>[2x]SNASKMSDVKCTSV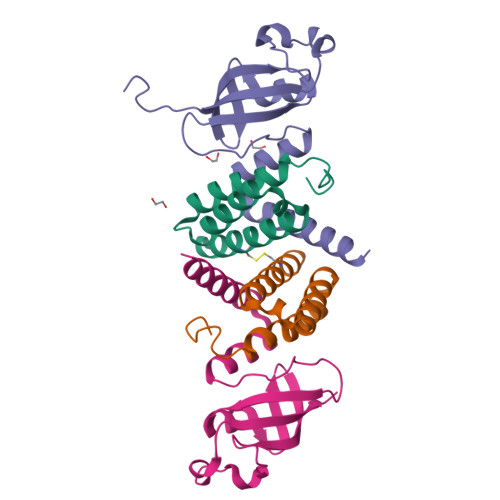VLLSVLQQLRVESSSKLWAQCVQLHNDILLAKDTTEAFEKMVSLLSVLLSMQGAVDINKLCEEMLDNRATLQ;>[2x]EDKRAKVTSAMQTMLFTMLRKLDNDALNNIINNARDGCVPLNIIPLTTAAKLMVVIPDYNTYKNTCDGTTFTYASALWEIQQVVDADSKIVQLSEISMDNSPNLAWPLIVTALRANSAVKLQ> NGIVPDAGHQGPDVSAVNGGTQVINIVTPNNEGISHNQYQDFNVGKPGAVFNNALE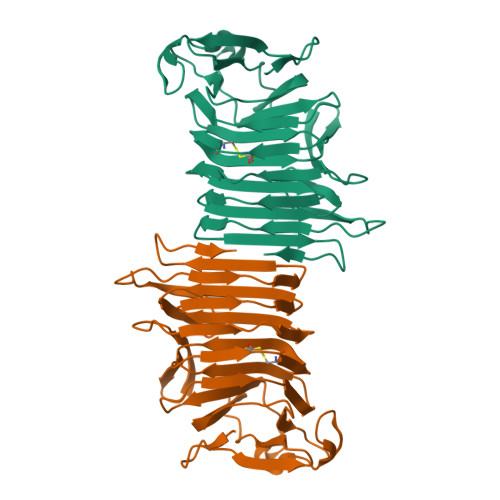AGQSQLAGHLNANSNLNGQAASLILNEVVSRNPSFLLGQQEVFGIAAEYVLSNPNGITCDGCGFINTSRSSLVVGNPLFENGQLKGYSTLNNTNLLSLGKNGLNTTGLLDLIAPRIDSRGKITAAEISAFTGQNTFSQHFDILSSQKPVSALDSYFFGSMQSGRIRIINTAEGSGVKLAGHHHHHH>LDNGLARTPTMGWLHWERFMCNLDCQEEPDSCISEKLFMEMAELMVSEGWKDAGYEYLCIDDCWMAPQRDSEGRLQADPQRFPHGIRQLANYVHSKGLKLGIYADVGNKTCAGFPGSFGYYDIDAQTFADW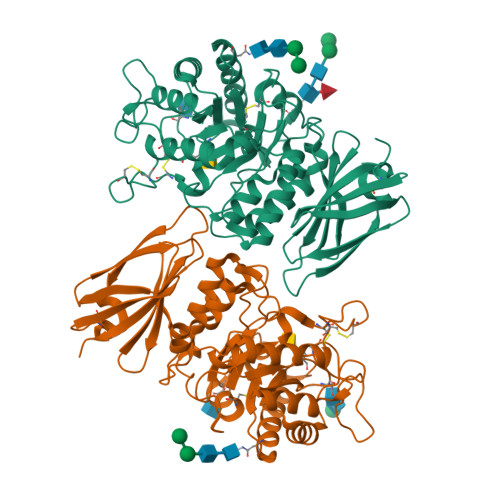GVDLLKFDGCYCDSLENLADGYKHMSLALNRTGRSIVYSCSWPAYMWPFQKPNYTEIRQYCNHWRNFADIDDSWKSIKSILDWTSFNQERIVDVAGPGGWNDPDMLVIGNFGLSWNQQVTQMALWAIMAAPLFMSNDLRHISPQAKALLQDKDVIAINQDPLGKQGYQLRQGDNFEVWERPLSGLAWAVAMINRQEIGGPRSYTIAVASLGKGVACNPACFITQLLPVKRKLGFYEWTSRLRSHINPTGTVLLQLENTMQMSLKDLLHHHHHH[2x]> GSPGISGGGGGSHIEGYECQPIFLNVLEAIEPGVVCAGHDNNQPDSFAALLSSLNELGERQLVHVVKWAKALPGFRNLHVDDQMAVIQYSWMGLMVFAMGWRSFTNVNSRMLYFAPDLVFNEYRMHKSRMYSQCVRMRHLSQEFGWLQITPQEFLCMKALLLFSIIPVDGLKNQKFFDELR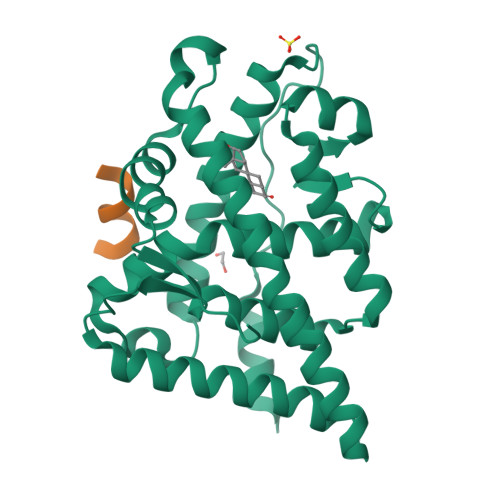MNYIKELDRIIACKRKNPTSCSRRFYQLTKLLDSVQPIARELHQFTFDLLIKSHMVSVDFPEMMAEIISVQVPKILSGKVKPIYFHTQ;> SRWQALFDDGTDTSR> FSSRTPVNENPDGVQYRRGFVTRHQVSGWRFVMRRIASGVALHDTRMLVDPLRTQSRAVLTGALIL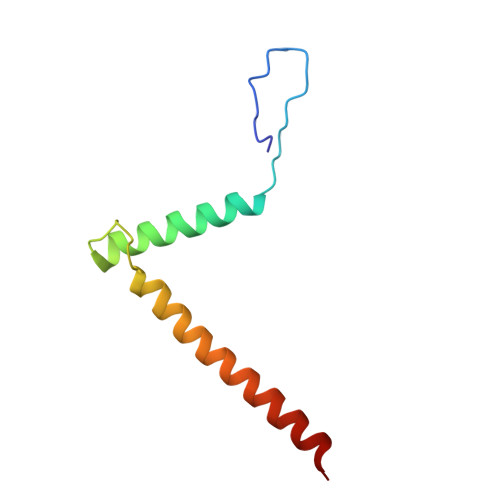VTGLVGCFIFSLFRP> DGLWDPTLPMIPSANIPGDPIAVVNQVLGISATSAQVTANMGRKFLEQLGILQPTDTGITNAPAGSAQGRIPRVYGRQASEYVIRRGMSQIGVPYSWGGGNAA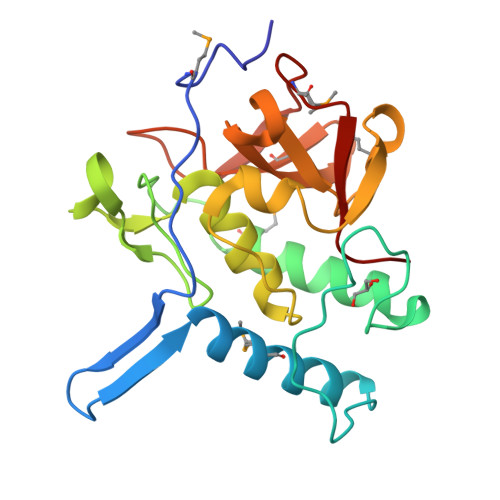GPSKGIDSGAGTVGFDCSGLVLYSFAGVGIKLPHYSGSQYNLGRKIPSSQMRRGDVIFYGPNGSQHVTIYLGNGQMLEAPDVGLKVRVAPVRTAGMTPYVVRYIEY>[2x]MRGSHHHHHHGSMSTTIQYNSNYADYSISSYLREWANNFGDIDQAPAETKDRGSFSGSSTLFSGTQYAIGSSHSNPEGMIAEGDLKYSF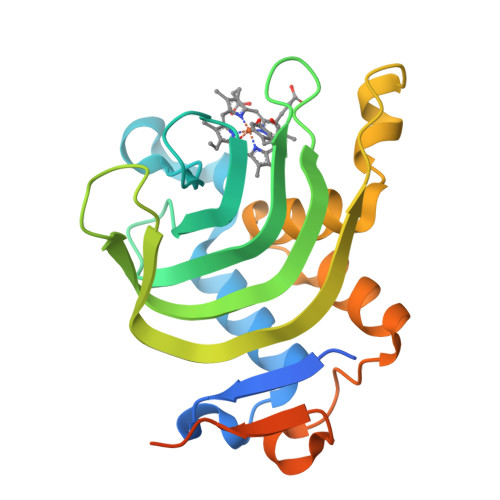MPQHTFHGQIDTLQFGKDLATNAGGPSAGKHLEKIDITFNELDLSGEFDSGKSMTENHQGDMHKSVRGLMKGNPDPMLEVMKAKGINVDTAFKDLSIASQYPDSGYMSDAPMVDTVGVMDSNDMLLAA>MLKREMNIADYDAELWQAMEQEKVRQEEHIELIASENYTSPRVMQAQGSQLTNKYAEGYPGKRYYGGCEYVDIVEQLAIDRAKELFGADYANVQPHSGSQANFAVYTALLEPGDTVLGMNLAHGGHLTHGSPVNFSGKLYNIVPYGIDATGHIDYADLEKQAKEHKPKMIIGGFSAYSGVVDWAKMREIADSIGAYLFVDMAHVAGLVAAGVYPNPVPHAHVVTTTTHKTLAGPRGGLILAKGGSEELYKKLNSAVFPGGQGGPLMHVIAGKAVALKEAMEPEFKTYQQQVAKNAKAMVEVFLERGYKVVSGGTDNHLFLVDLVDKNLTGKEADAALGRANITVNKNSVPNDPKSPFVTSGIRVGTPAITRRGFKEAEAKELAGWMCDVLDSINDEAVIERIKGKV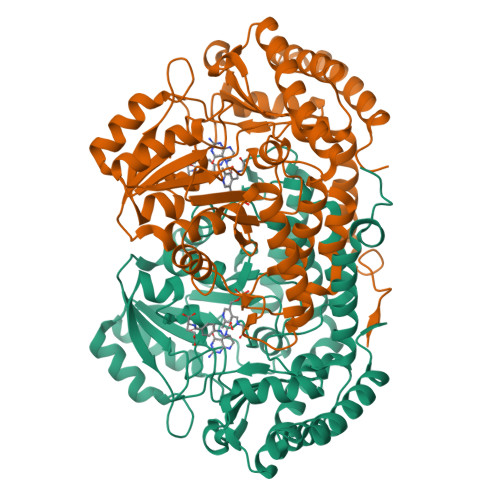LDICARYPVYA[4x]>[3x]MAGRWLDPLWAPGFLCVALILETASGAGDLSTKAHGHIQFSARGVNQTAMADCRAVCSLNTSDRCDFVKRNPDCHSEGGYLDYLKGIFCYFPPNLLPLAITLYVFWLLYLFLILGVTAAKFFCPNLSAISTSLKLSHNVAGVTFLAFGNGAPDIFSALVAFSDPRTAGLAIGALFGAGVLVTTVVAGGITILRPFMAASRPFLRDITFYMVAVFLTFTALYLGRITLVWALGYLGLYVFYVVTVIICTWVYQRQRSRSLVHSISETPELLTDSEEDQMSSNTNSYDYGEEYRPLLLGEETTGQILLQALNPLDYRKWRTQSISCKLLKVAKLPVEFLLLLTVPVVDPDKDDRNWKRPLNCLQLVISPLVLVLTLQSGVYGIYEIGGLLPVWAVVVIVGTALASVTFFATSNSEPPRLHWLFAFLGFLTSALWINAAATEVVNILRSLG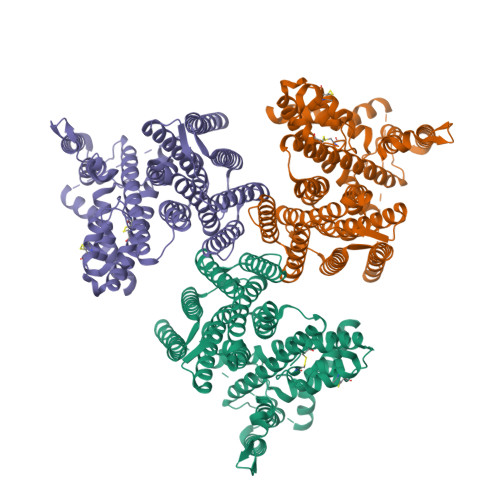VVFRLSNTVLGLTLLAWGNSIGDAFSDFTLARQGYPRMAFSACFGGIIFNILVGVGLGCLLQIVRSHASEVKLEPDGLLVWVLASALGLSLVFSLVSVPLQCFQLSKAYGLCLLLFYICFIVVVLLTEFGVIHLKAD> QKPQRPRRPASPISTIQPKANFDAQQFAGTWLLVAVGSAARFLQEQ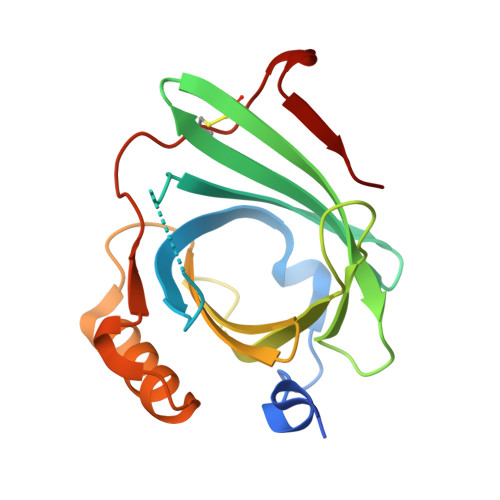GHRAEATTLHVAPQGTAMAVSTFRKLDGICWQVRQLWGDTGVLGRFLLQARGARGAVHVVVAETDYQSFAVLYLERAGQLSVKLYARSLPVSDSVLSGFEQRVQEAHLTEDQIFYFPKYGFCEAADQFHVLDEVRR2'-HYDROXY-1,1'-BIPHENYL-2-SULFINIC 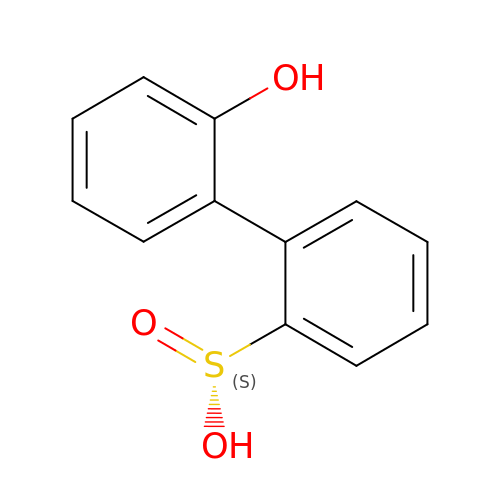ACID | C12 H10 O3 S | HPKSNFTYZHYEKV-UHFFFAOYSA-N>MRSRRVDVMDVMNRLILAMDLMNRDDALRVTGEVREYIDTVKIGYPLVLSEGMDIIAEFRKRFGCRIIADFKVADIPETNEKICRATFKAGADAIIVHGFPGADSVRACLNVAEEMGREVFLLTEMSHPGAEMFIQGAADEIARMGVDLGVKNYVGPSTAPERLSRLREIIGQDSFLISPG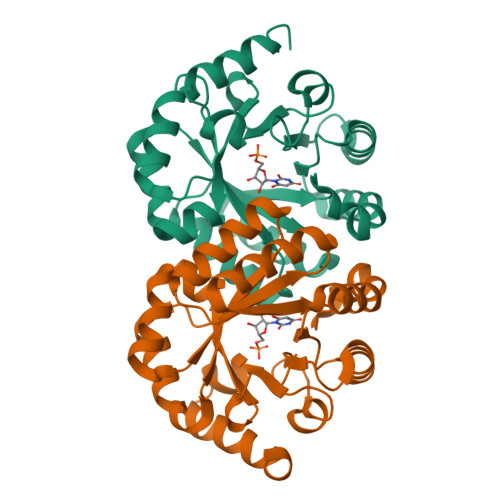VGAQGGDPGETLRFADAIIVGRSIYLADNPAAAAAGIIESIKDLLNP[2x]>[2x]MAEPLLVVGLGNPGANYAR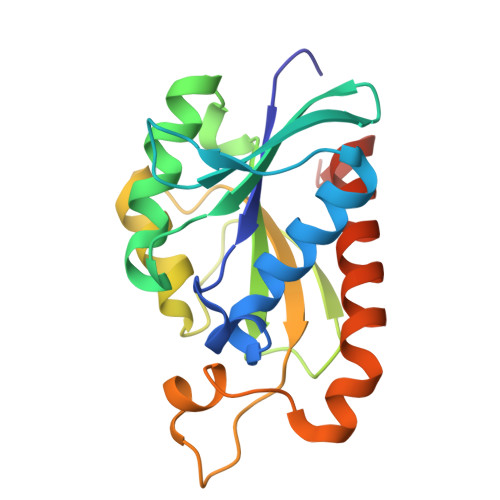TRHNLGFVVADLLAARLGAKFKAHKRSGAEVATGRSAGRSLVLAKPRCYMNESGRQIGPLAKFYSVAPANIIVIHDDLDLEFGRIRLKIGGGEGGHNGLRSVVAALGTKDFQRVRIGIGRPPGRKDPAAFVLENFTPAERAEVPTICEQAADATELLIEQGMEPAQNRVHAW The cytoplasmic-facing Lipid II is flipped to the periplasmic side of the membrane by a Lipid II flippase, after which the GlcNAc-MurNAc-pentapeptide moiety is incorporated into peptidoglycan and the lipid carrier is recycled. MurJ consists of 14 transmembrane helices (TMs), of which the first 12 are organized into two 6-TM bundles termed the N-lobe (TMs 1–6) and C-lobe (TMs 7–12). The N-lobe and C-lobe enclose a central cavity that is large and highly cationic, properties consistent with Lipid II transport. We determined four crystal structures of MurJTA: one structure in an outward-facing conformation to 1.8 Å resolution, and three structures in inward-facing conformations distinct from the published structure, resolved to 3.2, 3.0, and 2.6 Å, respectively.

One of the inward-facing structures exhibited a partially dilated membrane portal but was otherwise divergent from the rest of the inward-facing structures. Specifically, the C-lobe is bent with the cytoplasmic section swung ~15° towards the N-lobe. Conserved residues Pro260, Pro300, and Gly340 serve as hinges on TMs 8, 9, and 10, respectively. In contrast, re-arrangements in the N-lobe are restricted to the middle section of TM 2, which also bends inwards towards the central cavity. Notably, we observed unmodeled electron density peaks at the portal and at the central cavity above the thin gate. Although we cannot unambiguously assign the electron density to Lipid II, we hypothesized that this Glu57-Arg352 thin gate could occlude the flexible Lipid II molecule into the cavity prior to outward transition. Furthermore, a reliable in vitro lipid II flipping assay for MurJ is still not available despite attempts by us and others. Based on the abovementioned conformational changes, presence of the putative thin gate, and the unmodeled electron density, we tentatively assign this structure as an inward-occluded state of MurJ. In the inward-occluded state, Arg24 and Arg255 are brought into unusual proximity (just 2.9 Å apart at the closest) on top of the unmodeled electron density. Since such close contact between two arginine side chains would experience unfavorable repulsion, we reasoned that they could be stabilized by electrostatic interactions with Asp25 and the diphosphate moiety of Lipid II.

> MSILFSSILFSIATFFSRILGLFRDVLFAKYFGVSYELDAYFIAIMFPFFLRKVFGEGAMSSAFVPLYSEKSGEEKDKFLSSVINGFSLIILALVILSYFFPELIINLFGAGSSHETKILAKKLLLITSPSIYFIFLWAISYSILNTNNKFFWPALTPSISNITIIIGTFLSTKYGIISPTIGFLIGSILMFFSIIKSIIKHKYYFTIKHFPHFLKLFFPTFMTMVVSQINTVVDMNVVSFYDKGSISYLQYASRFYLLPYGLFAVSVSTVVLSKISNDRKNFNYHLNDALKTTLFFTIPSMVGLIFLSTPIIRFFYEHGAFTSKDTLITSKILIAYTLGLPFYGIYSTISRSYHAIKNTKTPFIAATIVSLSNIILDIIFGLKYGPIGVALATSIAGIIGVLYLLFSVKTFPIKDFLKISLNSLIMLFVIYLTDFTDNEFWFLIQILIGILVYLIFSSIFYRDLIRRFLYARKK>[4x]GSHMTNFVLGNAQIVDWPIVYSNDGFCKLSGYHRAEVMQKSSACSFMYGELTDKDTVEKVRQTFENYEMNSFEILMYKKNRTPVWFFVKIAPIRNEQDKVVLFLCTFSDITAFK

The KCNH family of voltage gated potassium channels includes the EAG (ether-a-go-go) channels, the ERG (eag related gene) channels and the ELK (eag like K+) channels; these channels have roles in cardiac repolarization, neuronal excitability, cell differentiation and tumor growth. A defining characteristic of KCNH channels is their large N- and C-terminal cytoplasmic regions. The N-terminus typically includes a Per-Arnt-Sim (PAS) domain, while the C-terminal region includes a domain that strongly resembles cyclic nucleotide binding domains, but which has been shown to have little affinity for cyclic nucleotides. As already stated, the role of PAS domains in KCNH channels is unknown; it is not known if these domains bind small ligands or mediate interactions between the channel and other proteins.

Crystals of mEAG PAS domain were obtained by removing the first 26 residues of the domain, which correspond to the disordered region detected in the hERG PAS structure. The asymmetric unit cell of mEAG PAS domain crystals contains four copies which, excluding the N- and C-termini, are very similar to each other (rmsd for main-chain atoms of residues 28 to132 varying between 0.2 and 0.6 Å). In contrast to dELK, all four structures in the asymmetric unit of the mEAG PAS domain show cavities that overlap with the one detected in hERG. The high resolution mEAG domain structures reveal multiple conformations for some side-chains, in particular in residues surrounding the cavity (S65, T86, I97, F109 and V111). Strikingly, the volume of the cavity in the mEAG PAS domain varies among the different models generated, from a minimum of ∼111 Å3 to a maximum of ∼136 Å3; the largest cavity has as maximum dimensions ∼8 6.5 6 Å. Only the conformers of V111 have any effect on the cavity properties, the remainder of the variation comes from adjustments in main-chain atoms. Unlike in hERG, the cavity in mEAG is isolated from the bulk solvent by a lid formed by a tyrosine side-chain (Y71); this residue occupies the same position as H70 in hERG (at the mouth of the cavity) but its larger side-chain occludes the opening. The residues that line the cavity defined in each conformer model vary but, in general, the polar face is determined by main-chain carbonyl groups from residues S65 and A66, as well as by the hydroxyl of the side-chain from Y71 and thiol groups from C67 and C128. The apolar face is formed by side-chains of apolar residues: V83, F87, I97, M99, V111, I113, and F130.>[3x]MILVTGGARSGKSRHAEALIGDAPQVLYIATSQILDDEMAARIQHHKDGRPAHWR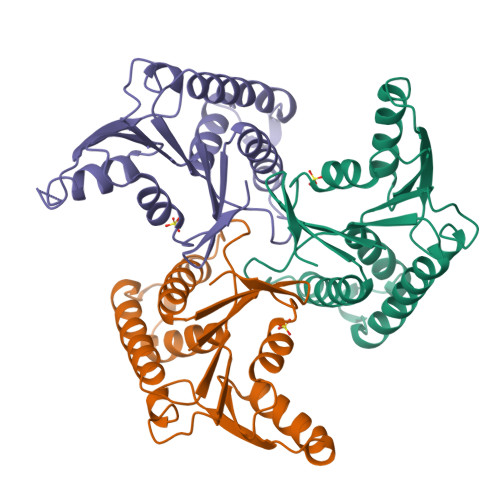TAECWRHLDTLITADLAPDDAILLECITTMVTNLLFALGGENDPEQWDYAAMERAIDDEIQILIAACQRCPAKVVLVTNEVGMGIVPENRLARHFRDIAGRVNQRLAAAADEVWLVVSGIGVKIK> MAAPAAEAPLSHVQQALAELAKPKDDPTRKHVCVQVAPAVRVAIAETLGLAPGATTPKQLAEGLRRLGFDEVFDTLFGADLTIMEQGSELLHRLTEHLEAHPHSDEPLPMFTSCCPGWIAMLEKSYPDLIPYVSSCKSPQMMLAAMVKSYLAEKKGIAPKDMVMVSIMPCTRKQ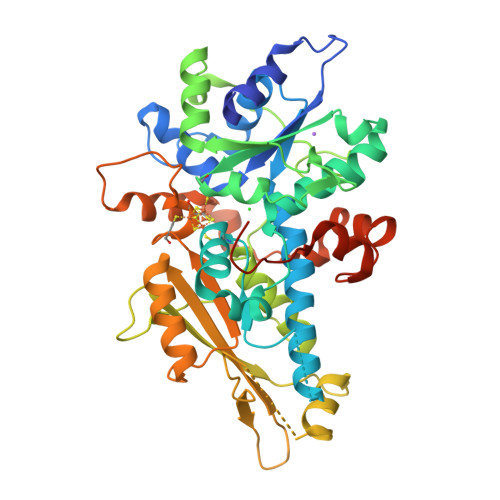SEADRDWFCVDADPTLRQLDHVITTVELGNIFKERGINLAELPEGEWDNPMGVGSGAGVLFGTTGGVMEAALRTAYELFTGTPLPRLSLSEVRGMDGIKETNITMVPAPGSKFEELLKHRAAARAEAAAHGTPGPLAWDGGAGFTSEDGRGGITLRVAVANGLGNAKKLITKMQAGEAKYDFVEIMACPAGCVGGGGQPRSTDKAITQKRQAALYNLDEKSTLRRSHENPSIRELYDTYLGEPLGHKAHELLHTHYVAGGVEEKDEKKSAWSHPQFEK>[6x]APVVNTAYGRVRGVRRELNNEILGPVVQFLGVPYATPPLGARRFQPPEAPASWPGVRNATTLPPACPQNLHGALPAIMLPVWFTDNLEAAATYVQNQSEDCLYLNLYVPTEDGPLTKKRDEATLNPPDTDIRDSGKKPVMLFLHGGSYMEGTGNMFDGSVLAAYGNVIVATLNYRLGVLGFLSTGDQAAKGNYGLLDQIQALRWLSENIAHFGGDPERITIFGSGAGASCVNLLILSHHSEGLFQKAIAQSGTAISSWSVNYQPLKYTRLLAAKVGCDREDSTEAVECLRRKSSRELVDQDVQPARYHIAFGPVVDGDVVPDDPEILMQQGEFLNYDMLIGVN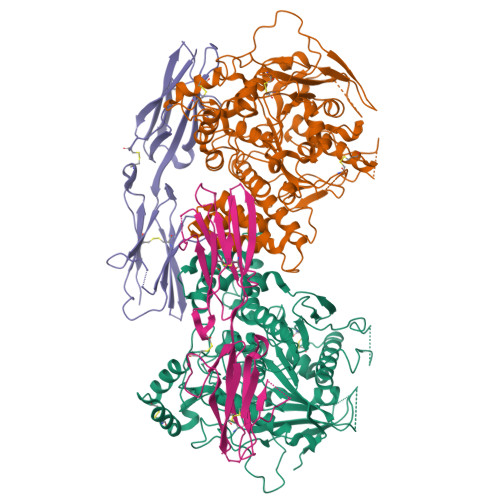QGEGLKFVEDSAESEDGVSASAFDFTVSNFVDNLYGYPEGKDVLRETIKFMYTDWADRDNGEMRRKTLLALFTDHQWVAPAVATAKLHADYQSPVYFYTFYHHCQAEGRPEWADAAHGDELPYVFGVPMVGATDLFPCNFSKNDVMLSAVVMTYWTNFAKTGDPNQPVPQDTKFIHTKPNRFEEVVWSKFNSKEKQYLHIGLKPRVRDNYRANKVAFWLELVPHLHNLHASTSHHHHHH;>VDYAPAQAQIVHAGQACVVKEDNISERVYTIREGDTLMLQCLVTGHPRPQVRWTKTAGSASDKFQETSVFNETLRIERIARTQGGRYYCKAENGVGVPAIKSIRVDVQYLDEPMLTVHQTVSDVRGNFYQEKTVFLRCTVNSNPPARFIWKRGSDTLSHSQDNGVDIYEPLYTQGETKVLKLKNLRPQDYASYTCQVSVRNVCGIPDKAITFRLTNTTGSASTSHHHHHH[6x]>SSQKKKKIAVMTSGGDSPGMNAAVRAVVRTGIHFGCDVFAVYEGYEGLLRGGKYLKKMAWEDVRGWLSEGGTLIGTARSMEFRKREGRRQAAGNLISQGIDALVVCGGDGSLTGADLFRHEWPSLVDELVAEGRFTKEEVAPYKNLSIVGLVGSIDNDMSGTDSTIGAYSALERICEMVDYIDATAKSHSRAFVVEVMGRHCGWLALMAGIATGADYIFIPERAVPHGKWQDELKEVCQRHRSKGRRNNTIIVAEGALDDQLNPVTANDVKDALIELGLDTKVTILGHVQRGGTAVAHDRWLATLQGVDAVKAVLEFTPETPSPLIGILENKIIRMPLVESVKLTKSVATAIENKDFDKAISLRDTEFIELYENFLSTTVKDDGSELLPVSDRLNIGIVHVGAPSAALNAATRAATLYCLSHGHKPYAIMNGFSGLIQTGEVKELSWIDVENWHNLGGSEIGTNRSVASEDLGTIAYYFQKNKLDGLIILGGFEGFRSLKQLRDGRTQHPIFNIPMCLIPATVSNNVPGTEYSLGVDTCLNALVNYTDDIKQSASATRRRVFVCEVQGGHSGYIASFTGLITGAVSVYTPEKKIDLASIREDITLLKENFRHDKGENRNGKLLVRNEQASSVYSTQLLADIISEASKGKFGVRTAIPGHVQQGGVPSSKDRVTASRFAVKCIKFIEQWNKKNEASPNTDAKVLRFKFDTHGEKVPTVEHEDDSAAVICVNGSHVSFKPIANLWENETNVELRKGFEVHWAEYNKIGDILSGRLKLRAEVAALAAENK[4x];>RPQKAIAVMTSGGDAPGMNSNVRAIVRSAIFKGCRAFVVMEGYEGLVRGGPEYIKEFHWEDVRGWSAEGGTNIGTARCMEFKKREGRLLGAQHLIEAGVDALIVCGGDGSLTGADLFRSEWPSLIEELLKTNRISNEQYERMKHLNICGTVGSIDNDMSTTDATIGAYSALDRICKAIDYVEATANSHSRAFVVEVMGRNCGWLALLAGIATSADYIFIPEKPATSSEWQDQMCDIVSKHRSRGKRTTIVVVAEGAIAADLTPISPSDVHKVLVDRLGLDTRITTLGHVQRGGTAVAYDRILATLQGLEAVNAVLESTPDTPSPLIAVNENKIVRKPLMESVKLTKAVAEAIQAKDFKRAMSLRDTEFIEHLNNFMAINSADHNEPKLPKDKRLKIAIVNVGAPAGGINSAVYSMATYCMSQGHRPYAIYNGWSGLARHESVRSLNWK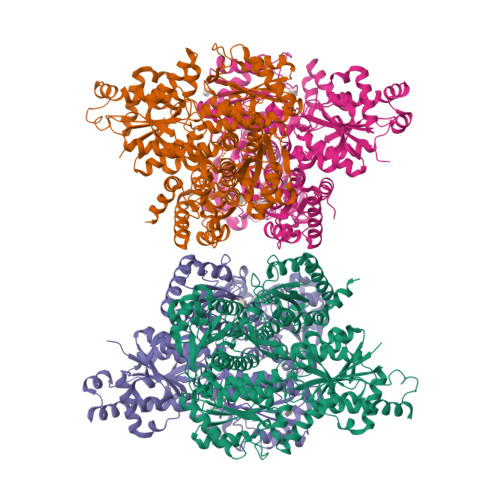DMLGWQSRGGSEIGTNRVTPEEADLGMIAYYFQKYEFDGLIIVGGFEAFESLHQLERARESYPAFRIPMVLIPATLSNNVPGTEYSLGSDTALNALMEYCDVVKQSASSTRGRAFVVDCQGGNSGYLATYASLAVGAQVSYVPEEGISLEQLSEDIEYLAQSFEKAEGRGRFGKLILKSTNASKALSATKLAEVITAEADGRFDAKPAYPGHVQQGGLPSPIDRTRATRMAIKAVGFIKDNQAAIAEARAAEENFNADDKTISDTAAVVGVKGSHVVYNSIRQLYDYETEVSMRMPKVIHWQATRLIADHLVGRKRVD[4x]>MARFNAAFTRIKIMFSRIRGLISCQSNTQTIAPTLSPPSSGHVSFAGIDYPLLPLNHQTPLVFQWFERNPDRFGQNEIPIINTQKNPYLNNIINAAIIEKERIIGIFVDGDFSKGQRKALGKLEQNYRNIKVIYNSDLNYSMYDKKLTTIYLENITKLEAQSASERDEVLLNGVKKSLEDVLKNNPEETLISSHNKDKGHLWFDFYRNLFLLKGSDAFLEAGKPGCHHLQPGGGCIYLDADMLLTDKLGTLYLPDGIAIHVSRKDNHVSLENGIIAVNRSEHPALIKGLEIMHSKPYGDPYNDWLSKGLRHYFDGSHIQDYDAFCDFIEFKHENIIMNTSSLTASSWR[4x]

The non-LEE encoded effector protein B (NleB) has GT activity and inhibits NF-κB activation by transferring N-acetyl glucosamine (GlcNAc) to host death domain-containing proteins and to glyceraldehyde 3-phosphate dehydrogenase (GAPDH). The glycosylation target is an arginine residue, which was unexpected because the guanidine group of arginine is nucleophilically poor at physiological pH. The T3SS effectors SseK1 and SseK2 from Salmonella typhimurium SL1344 are NleB orthologs that behave as NleB1-like GTs, although they differ in protein substrate specificity. Here, by using a combination of X-ray crystallography, STD-NMR, enzyme kinetics, molecular dynamics simulations, and in vivo experiments, we show that these enzymes are GT-A fold retaining GTs that most likely follow an SNi mechanism.

Based on the complexes of SseK2 with UDP and UDP-GlcNAc, we identified the donor-substrate binding mode and substrate-mediated conformational changes. The uridine group has an aromatic ring tethered by Phe203 and Trp65 through π-π stacking, water-mediated indirect hydrogen bonds (backbones of Arg68 and Ser346), and hydrogen bonding with the Phe66 backbone. The GlcNAc moiety of UDP-GlcNAc establishes hydrogen bond interactions with Asp204, Arg207, Asp239, and Arg348. The acetyl group of GlcNAc stabilizes the manganese ion by water-mediated hydrogen bonds. An octahedral molecular geometry was visualized for the manganese ion coordinated to six oxygens from the UDP pyrophosphate, Asp241, Ser340, Asn338, and a water molecule. The SseK2 structure undergoes a dramatic conformational change induced by donor-substrate binding. After UDP-GlcNAc binds to the active site, the α10 helix is tilted towards the UDP-GlcNAc by ~ 3.5° and the C-terminal lid domain covers up the active site to stabilize the bound substrate and to restrict the accessibility of water molecules. The closure of the C-terminal lid in the presence of UDP-GlcNAc determines a closed conformation for this family of enzymes. In the SseK2-UDP-GlcNAc crystal structure (chain D), Asn272 (corresponding to Asn256SseK1) is closer to the C1 anomeric carbon of UDP-GlcNAc (5.1 Å) as compared to Glu271 (5.6 Å). These data indicate that the Asn272 may play an important role in binding and catalysis.5,6,8-trimethoxy-1,4-dimethylquinolin-2(1H)-one | C14 H17 N O4 | 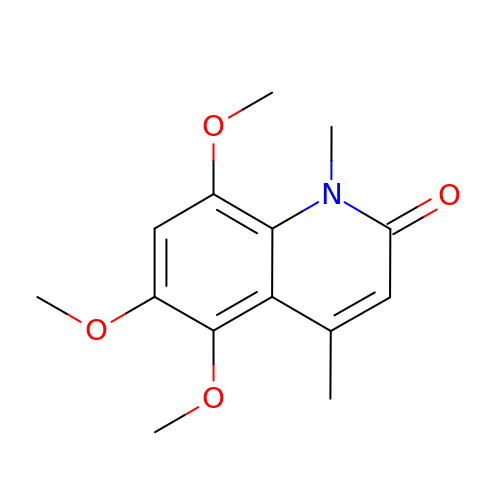PJUNWPXRLZUYPB-UHFFFAOYSA-N> MKYGYFDNDNREYVITRPDVPAPWTNYLGTEKFCTVISHNAGGYSFYNSPEYNRVTKFRPNATFDRPGHYVYLRDDDSGDYWSISWQPVAKSLDEAQYQIRHGLSYSKFQCDYNGIHARKTLFVPKGEDAEIWDVVIKNTSDQVRTISAFSFVEFSFSHIQSDNQNHQMSLYSAGTAYRPGLIEYDLYYNTDDFEGFYYLASTFDPDSYDGQRDRFLGLYRDEANPLAVEQGRCSNSAQTCYNHCGSLHKQFTLQPGEEIRFAYILGIGKGNGERLREHYQDVANIDAAFAAIKAHWDERCAKFQVKSPNQGLDTMINAWTLYQAETCVVWSRFASFIEVGGRTGLGYRDTAQDAISVPHANPEMTRKRIVDLLRGQVKAGYGLHLFDPDWFDPEKEDVAPSKSPTVVPTPSDEDKIHGIKDTCSDDHL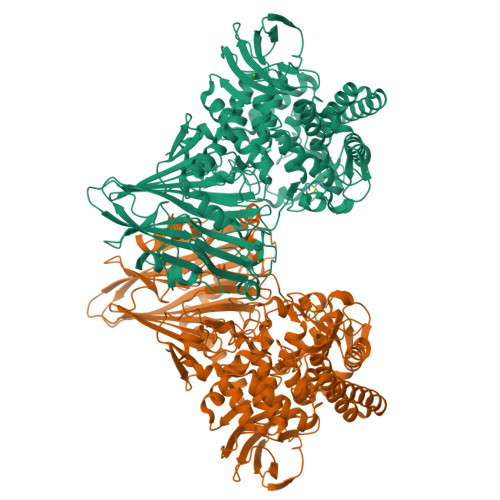WLIPTICKYVMETGETSFFDQMIPYADGGEASVYEHMKAALDFSAEYVGQTGICKGLRADWNDCLNLGGGESSMVSFLHFWALQEFIDLAKFLGKDQDVNTYTEMAANVREACETHLWDDEGGWYIRGLTKNGDKIGTAQQQEGRVHLESNTLAVLSGLASQERGEQAMDAVDEHLFSPYGLHLNAPSFSTPNDDIGFVTRVYQGVKENGAIFSHPNPWAWVAETKLGRGDRAMKFYDALNPYNQNDIIEKRIAEPYSYVQFIMGRDHQDHGRANHPWLTGTSGWAYFAVTNYILGVQSGFTGLSVDPCIPSDWPGFEVTRQWRGATYHIQVENPDHVSKGVKSITLNGAPIQGRIPPQAQGSDNQVVVVLGHHHHHH> SSCCSSEDRANVMHNWDAAWSAAYSDRRVALAQAVFASLFSRDAAAQGLFSGVSADNPDSADFRAHCVRVVNGLDVAINMLNDP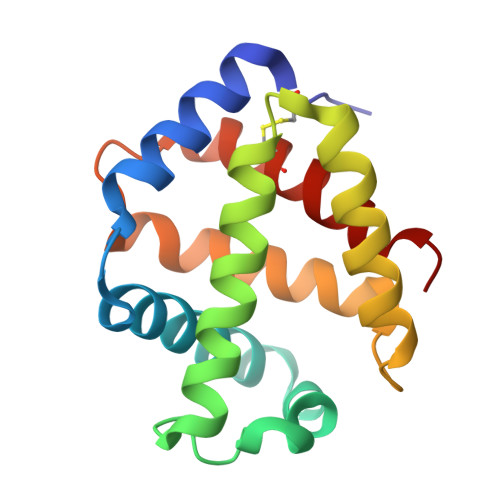AVLNEQLAHLSAQHQARAGVAAAHFDVMAEAFAEVMPQVSSCFSSDSWNRCFARIANGISAGL> SEILNN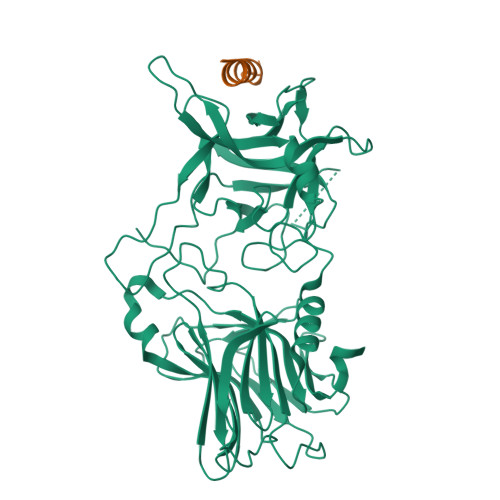IILNLRYKDNNLIDLSGYGAKVEVYDGVELNDKNQFKLTSSANSKIRVTQNQNIIFNSVFLDFSVSFWIRIPKYKNDGIQNYIHNEYTIINCMKNNSGWKISIRGNRIIWTLIDINGKTKSVFFEYNIREDISEYINRWFFVTITNNLNNAKIYINGKLESNTDIKDIREVIANGEIIFKLDGDIDRTQFIWMKYFSIFNTELSQSNIEERYKIQSYSEYLKDFWGNPLMYNKEYYMFNAGNKNSYIKLKKDSPVGEILTRSKYNQNSKYINYRDLYIGEKFIIRRKSNSQSINDDIVRKEDYIYLDFFNLNQEWRVYTYKYFKKEEEKLFLAPISDSDEFYNTIQIKEYDEQPTYSCQLLFKKDEESTDEIGLIGIHRFYESGIVFEEYKDYFCISKWYLKEVKRKPYNLKLGCNWQFIPKDEGWTEPP;> EDMFAKLKDKFFNEINK>GPERTFIMVKPDGVQRGLVGEVIQRFERRGYKLVAIKMMHASEQLLQTHYEALKSLSFFPKLVAYMSSGPVVPMVFEGRKVVENGRTMLGATKPEASCPGSIRGDYCQDVGRNVVHGSDSTESANREINLWFSPQELCQYKQAVDPWIH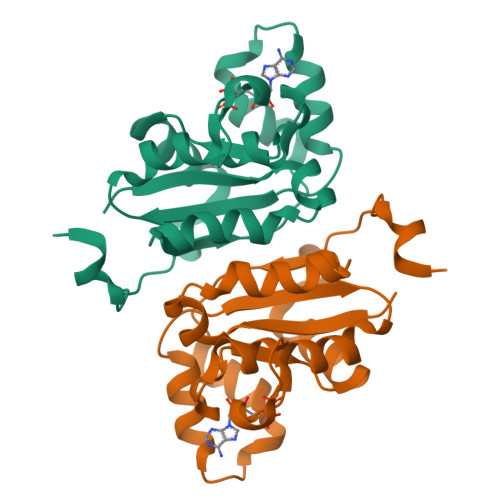E[2x]>[4x]MGPAPRVLELFYDVLSPYSWLGFEVLCRYQHLWNIKLKLRPALLAGIMKDS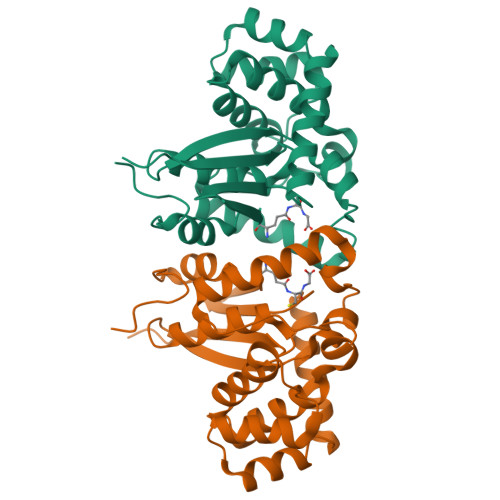GNQPPAMVPHKGQYILKEIPLLKQLFQVPMSVPKDFFGEHVKKGTVNAMRFLTAVSMEQPEMLEKVSRELWMRIWSRDEDITESQNILSAAEKAGMATAQAQHLLNKISTELVKSKLRETTGAACKYGAFGLPTTVAHVDGKTYMLFGSDRMELLAYLLGEKWMGPVPPTLNARL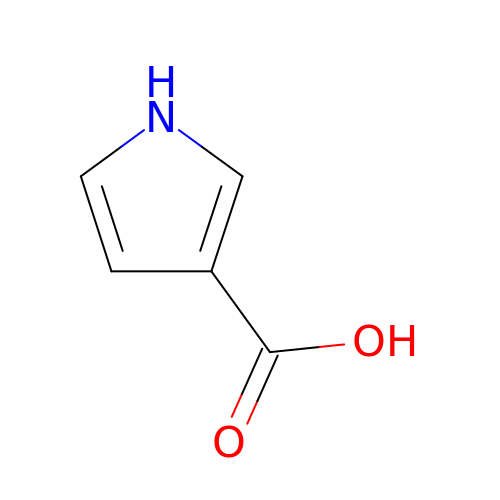1H-pyrrole-3-carboxylic acid | C5 H5 N O2 | DOYOPBSXEIZLRE-UHFFFAOYSA-N4-ethyl-2-oxoglutarate 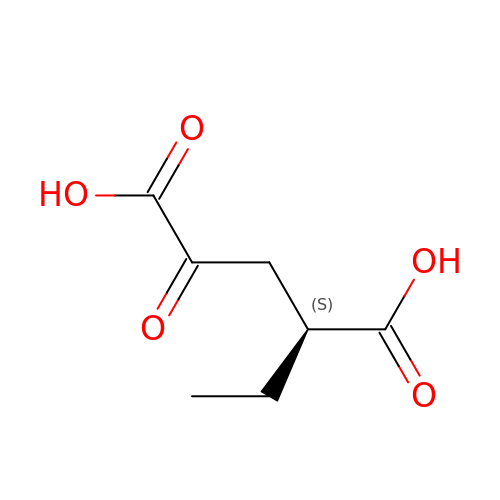| C7 H10 O5 | RLMBQTSJQCNDCM-BYPYZUCNSA-N>[12x]MNSQLTLRALERGDLRFIHNLNKELARY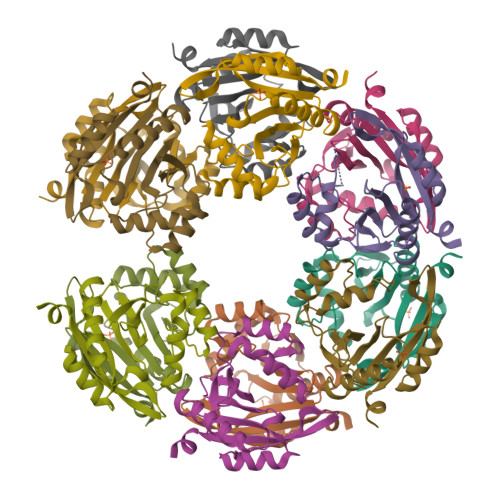EYWFEEPYESFDELEELYNKHIHDNAERRFVVEDAQKNLIGLVELIEINYIHRSAEFQIIIAPEHQGKGFARTLINRALDYSFTILNLHKIYLHVAVENPKAVHLYEECGFVEEGHLVEEFFINGRYQDVKRMYILQSKYLNRSE High expression of PSMαs, which are four peptides of about 20-residues in length, increases virulence potential of methicillin-resistant S. aureus (MRSA). Amyloid aggregation plays roles in PSM activities in S. aureus. In the present study, we investigated the structure-function relationships of PSMαs and their short truncations.

We found that the LFKFFK segment from PSMα3, identified as fibril-forming by computational methods and which indeed forms fibrils, shows dose-dependent antibacterial activity against Gram-positive Micrococcus luteus and Staphylococcus hominis, but is nontoxic to S. aureus, the secreting bacterium. We obtained two atomic resolution structures of LFKFFK; both revealed a departure from cross-β fibrils and atypical amyloid architectures. One polymorph was fundamentally different from steric-zippers, displaying no dry interface between pairs of β-sheets. Instead, hexamers of β-sheets formed cylindrical channels running along the fibril-like structure, effectively yielding nanotubes. The hexameric configuration lacks the tight interdigitation of β-sheets characteristic of canonical cross-β fibrils, such as PSMα4-IIKVIK and eukaryotic steric-zipper amyloid segments, resulting in a smaller solvent-accessible surface area buried and lower shape complementarity at the interface between the β-sheets. Moreover, the cylindrical architecture of LFKFFK polymorph I is reminiscent of that displayed by a polymorph of amyloid-β fibrils, and a HET-s prion fragment. The FF motif is present in the LFKFFK segment, and the hexameric structure of LFKFFK resembles the FF nanotubes. This farther support the role of self-assembly in antibacterial activity and specifically the hexamric arrangement that forms channels along the fibril axis.

> LFKFFK> TDTTNSIKHVISPLARQTLQDRDLTRPVAGKRPIRLLPWLQVVKIGGRVMDRGADAILPLVEELRKLLPEHRLLILTGAGVRARHVFSVGLDLGLPVGSLAPLAASEAGQNGHILAAMLASEGVSYVEHPTVADQLAIHLSATRAVVGSAFPPYAHHEFPGSRIPPHRADTGAFLLADAFGAAGLTIVENVDGIYTADPNGPDRGQARFLPETSATDLAKSEGPLPVDRALLDVMATARHIERVQVVNGLVPGRLTAALRGEHVGTLIRTGVRPA;> ANSTAELEELLMQRSLTDPQLQAAAAAAADFRILPDATVIKIGGQSVIDRGRAAVYPLVDEIVAARKNHKLLIGTGAGTRAR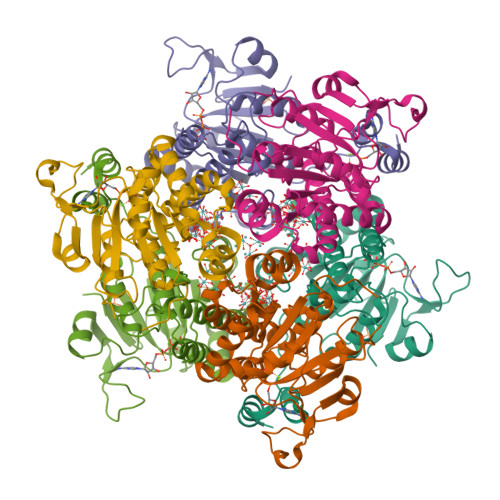HLYSIAAGLGLPAGVLAQLGSSVADQNAAMLGQLLAKHGIPVVGGAGLSAVPLSLAEVNAVVFSGMPPYKLWMRPAAEGVIPPYRTDAGCFLLAEQFGCKQMIFVKDEDGLYTANPKTSKDATFIPRISVDEMKAKGLHDSILEFPVLDLLQSAQHVREVQVVNGLVPGNLTRALAGEHVGTIITAS Pseudomonas species and other aerobic bacteria have a biotin-independent malonate decarboxylase that is crucial for their utilization of malonate as the sole carbon and energy source. MdcA, MdcC, MdcD, and MdcE form the 140 kD MDC holoenzyme, with 1:1:1:1 stoichiometry among the four subunits. The malonyl-ACP is decarboxylated in the second step of the reaction to regenerate acetyl-ACP, which is catalyzed by MdcD (30 kD) and MdcE (28 kD).

We determined the crystal structure of the P. aeruginosa MdcD–MdcE complex at 1.86 Å resolution by the selenomethionyl single-wavelength anomalous diffraction method. The two copies of the MdcD–MdcE complex in the asymmetric unit have essentially the same conformation, with overall rms distance of 0.4 Å between their equivalent Cα atoms. The structures of the MdcD and MdcE subunits have the crotonase fold, with a β–β–α motif that is repeated four times in its core (β–β–α superhelix). The two subunits are related by a rotation of 173° in this complex, suggesting pseudo two-fold symmetry between them. The A. calcoaceticus MdcD–MdcE complex was reported to be a 2:2 hetero-tetramer in solution, and the MdcD subunit itself could also dimerize. In contrast, the P. aeruginosa MdcD–MdcE complex is a 1:1 hetero-dimer in solution based on our gel filtration data, and a 2:2 hetero-tetramer was not observed in the crystal either. The structural overlay with the S. aureus CT indicates that the C-terminal helices (α8A and α8B) of MdcD clash with the second copy of the S. aureus CT and therefore the MdcD–MdcE complex is incompatible with the CT hetero-tetramer, which may explain why Pseudomonas MdcD–MdcE is a 1:1 complex. In fact, this helix and the following residues are mostly disordered in the malonate complex and MdcD–MdcE alone.

>MGSSHHHHHHSQDPNSMSQPFASRGLAWFQALAGSLAPRPGDPASLRVADAELDGYPVRFLAVVPDPDNPFPRARQGEVGLLEGWGLAAAVDEALEADREAPRKRALLAIVDVPSQAYGRREEALGIHQALAGAVDAYARARLAGHPLIGLLVGKAMSGAFLAHGYQANRLIALHDPGVMVHAMGKAAAARITLRSVEELEALAAKVPPMAYDIDSYASLGLLWRTLPVETVEVPSTADLVRVRTCLGEALADILGGPRDLGGRLGAANREASARVRRLLREQW[2x];>MTDVARLLALRSFTELGARQRARALLDAGSFRELLDPFAGVQSPWLERQGIVPQADDGVVVARGLLDGQPAVLAAIEGAFQGGSLGEVSGAKIAGALELAAEDNRNGVPTRALLLLETGGVRLQEANLGLAAIAEIQAAIVDLQRYQPVVAVIAGPVGCFGGMSIAAGLCSYVLVTREARLGLNGPQVIEQEAGIAEYDSRDRPFIWSLTGGEQRFASGLADAYLADDLDEVRTSVLAYFAKGLPARPRCRRAEDYLRRLGDLDTAEQPDAAGVRRLYQGLGQGDAT[2x]> HHHHHHSSGLVPRGSHMSGEKRDVLAELGLGDLRPYLRSIGDKDRIFPKAHRIEVVFLVRAANYLLLRTEGAGTINMTTLEYSGGAMEVPVIQPQKLMAVTRRQMLQLLREYRDSLDEVSKRWLVQEVIGKAKDLGFKKVSEEWNCTIQPPLAEFGEKATDIGMDGFCPHCTIFGAALTEQHNEKFGGLSIGIKTRVRFDPAFATQRRITPETHNKVTEGHLSMTGQALFSEVHVEPGTVFIGRAELVDLTEPELVATLYSLATLRELGGRSGIYGTVRVE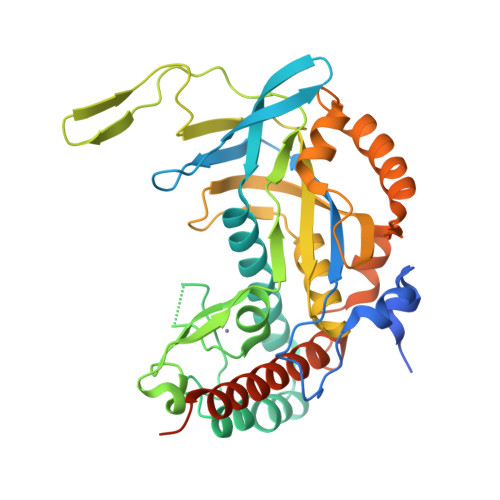ILGVKAGKYASTTAYDLAAENAGKGYEEVKKNLKERLEKLGFTPVDNSKLLAAVDHKDPNGLFKDLWRSSIDFAEKMVKWVEELKGGGQKGSGKKSRSKKAEPEESEEE> MAQRQFFGLTYNFYGQPAPLFDLNDLQELAGCYARPWTSRFSHLAISTGSLPVWSARYPSVASRNIVVNTLLGAHLNPFAGGQITSHQGITWRDPVLSSLAPVPAIQPPPVWAVAENVLLDSNNYPTYVLNLSSMWPINQDVHIMTMWALSDQGPIYHLEVPVDPMPAATTAALMAYTGVPIAHLAQTAYRFAGQLPQSPDSTMVSTIRWLSAIWFGSLTGRLNRSRTCNGFYFEFAKPALNPDQAVLKWNDGARAAPPAAAQSSYIRCISPHWQHQIVEVAGALMSQSVTAVTGLPALID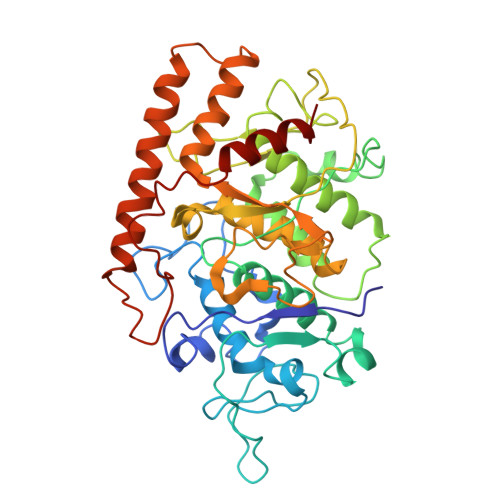EATLPAWSQGVANLTGNGQGVVPCLDYNPVPMAAARHLQWRQDGLITAAQEAQLNNDYTAYALTIERHLTAMLVANPIAAGRMPIQPFNAADFGQAGQTAAAVALAQAMFV> PPPALPP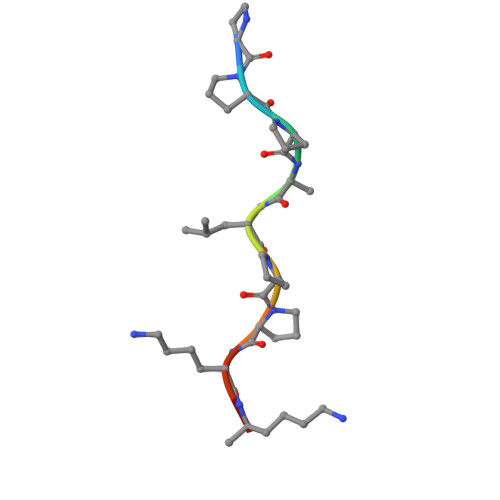KKR> GPNLFVALYDFVASGDNTLSITKGEKLRVL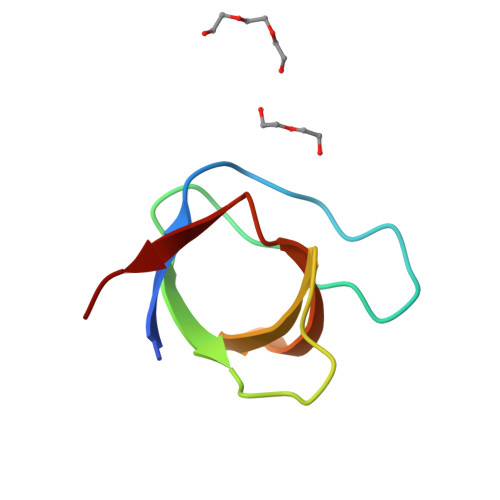NNTENGEWCEAQTKNGQGWVPSNYITPVN1-[3-amino-6-(3-methoxyphenyl)pyrazin-2-yl]piperidine-4-carboxylic acid | C17 H20 N4 O3 | 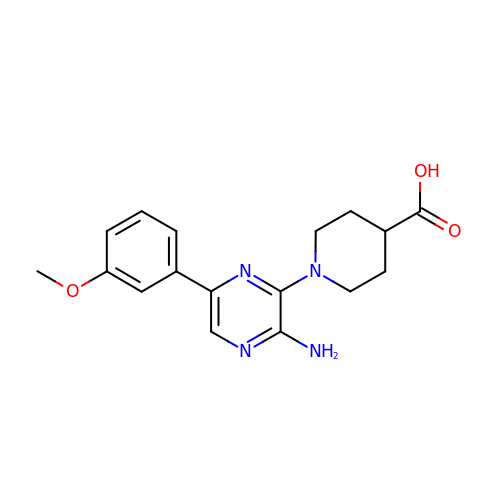DXJSLXVHZRWEMR-UHFFFAOYSA-N> MEALWLWIGFVGMLLGTLYFAFLLTNAPEGTRYFFVITATITGIAAIAYLVMATGSGSTVLPDGREFYWARYIDWVITTP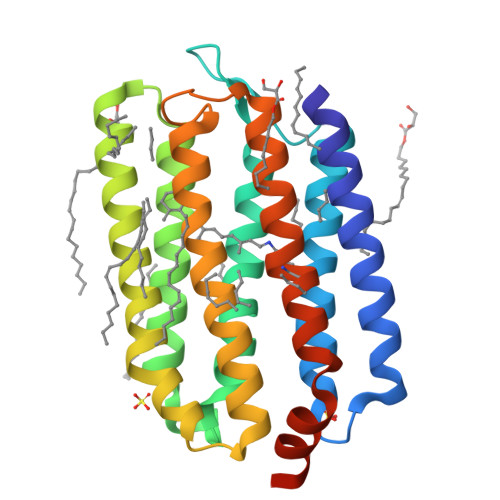LLLLDLCLLALADPRRNVTFIASLIALDVVMILTGLWAGATVNVAGRAILFIISTAAFIGVLYLLVSRLFAEASRRTPAVAQIFRTLAVLTIVLWICYPIVWLIGTEGFGAVSLSVEVFLFMVLDLLAKVGFGLLLLSSRQALSDIGSGAVAGTARRVA>[2x]MQDCGLPPDVPNAQPALEGRTSFPEDTVITYKCEESFVKIPGEKDSVICLKGSQWSDIEEFCNRSCEVPTRLNSASLKQPYITQNYFPVGTVVEYECRPGYRREPSLSPKLTCLQNLKWSTAVEFCKKKSCPNPGEIRNGQIDVPGGILFGATISFSCNTGYKLFGSTSSFCLISGSSVQWSDPLPECREIYCPAPPQIDNGIIQGERDHYGYRQSV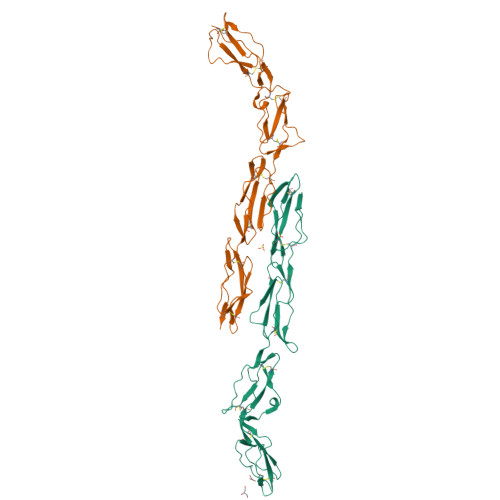TYACNKGFTMIGEHSIYCTVNNDEGEWSGPPPECRGC> FLKFVILHAEDDTDEALRVQNLLQDDFGIKPGIIFAEMPHGRQHLQNLDDAVNGSAWTILLLTENFLRDTWCNFQFY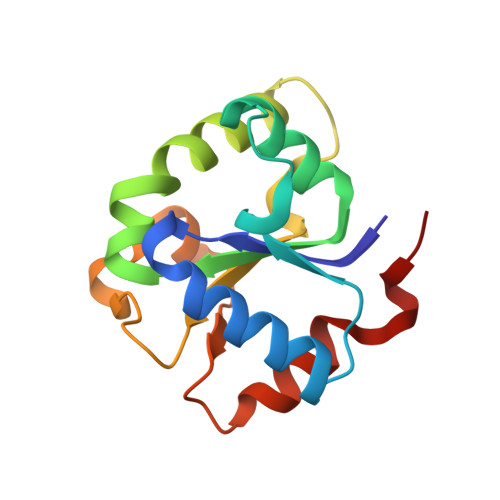TSLMNSVNRQHKYNSVIPMRPLNNPLPRERTPFALQTINALEEESRGFPTQVERIFQESVYKT>[2x]VTGDTDQPIHIESDQQSLDMQGNVVTFTGNVIVTQGTIKINADKVVVTRPGGE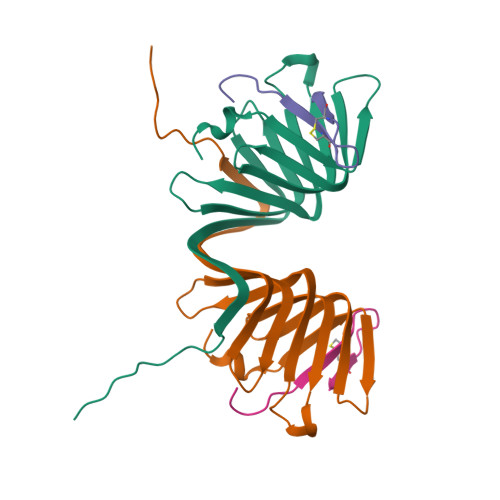QGKEVIDGYGKPATFYQMQDNGKPVEGHASQMHYELAKDFVVLTGNAYLQQVDSNIKGDKITYLVKEQKMQAFSDKGKR;>[2x]GSKPVPIIACNRKTGKCTRI>[2x]MRVAMISMHTSPLQQPGTGDSGGMNVYILSTATELAKQGIEVDIYTRATRPSQGEIVRVAENLRVINIAAGPYEGLSKEELPTQLAAFTGGMLSFTRREKVTYDLIHSHYWLSGQVGWLLRDLWRIPLIHTAHTLAAVKNSYRDDSD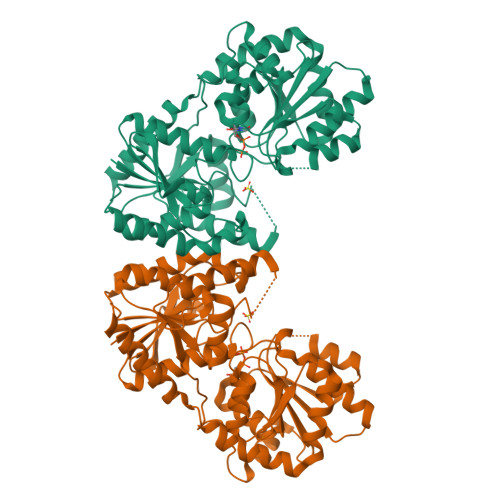TPESEARRICEQQLVDNADVLAVNTQEEMQDLMHHYDADPDRISVVSPGADVELYSPGNDRATERSRRELGIPLHTKVVAFVGRLQPFKGPQVLIKAVAALFDRDPDRNLRVIICGGPSGPNATPDTYRHMAEELGVEKRIRFLDPRPPSELVAVYRAADIVAVPSFNESFGLVAMEAQASGTPVIAARVGGLPIAVAEGETGLLVDGHSPHAWADALATLLDDDETRIRMGEDAVEHARTFSWAATAAQLSSLYNDAIANENVDGETHHGLEHHHHHH> MSFVKDFKPQALGDTNLFKPIKIGNNELLHRAVIPPLTRMRALHPGNIPNRDWAVEYYTQRAQRPGTMIITEGAFISPQAGGYDNAPGVWSEEQMVEWTKIFNAIHEKKSFVWVQLIVLGWAAFPDNLARDGLRYDSASDNVFMDAEQEAKAKKANNPQHSLTKDEIKQYIKEYVQAAKNSIAAGADGVEIHSANGYLLNQF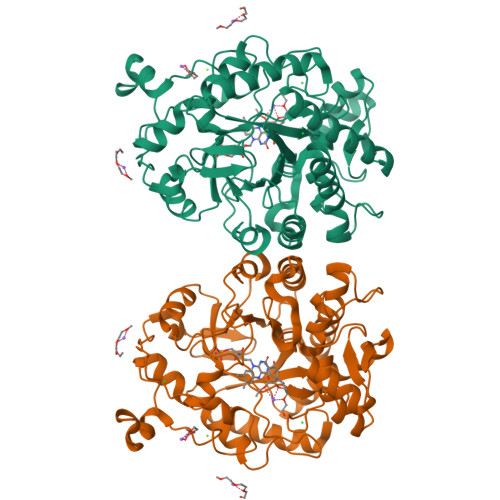LDPHSNTRTDEYGGSIENRARFTLEVVDALVEAIGHEKVGLRLSPYGVFNSMSGGAETGIVAQYAYVAGELEKRAKAGKRLAFVHLVEPRVTNPFLTEGEGEYEGGSNDFVYSIWKGPVIRAGNFALHPEVVREEVKDKRTLIGYGRFFISNPDLVDRLEKGLPLNKYDRDTFYQMSAHGYIDYPTYEEALKLGWDKK>[4x]SIGVSDGLLSYIKNENENKGFLGIYGFFTGADKNIEKAT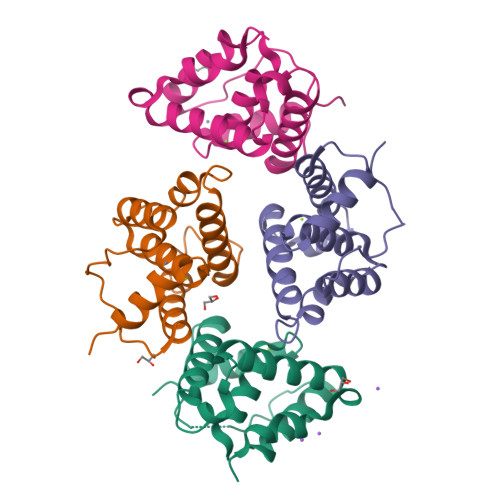LYKNLIAKYQNNHFISLIILSALVSDSKTPLMTQYLVGYLDFPSKALLANKITELLLKELENPDMREILGSRLATDVIEELETKIIRYIHNPAGSDIHSTLNLWTADKIKAATNSSLTI>[2x]M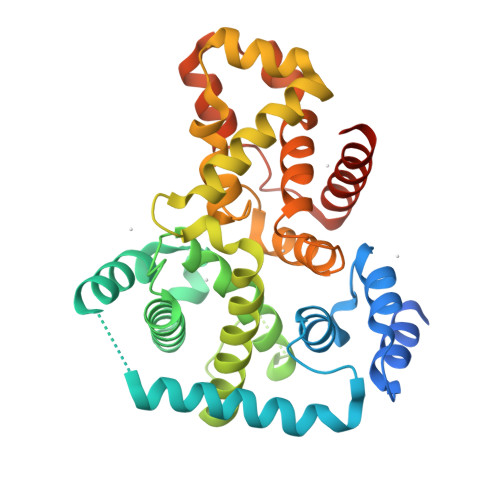HHHHHHSSGRENLYFQGSEREASRLDKFKQLLAGPNTDLEELRRLSWSGIPKPVRPMTWKLLSGYLPANVDRRPATLQRKQKEYFAFIEHYYDSRNDEVHQDTYRQIHIDIPRMSPEALILQPKVTEIFERILFIWAIRHPASGYVQGINDLVTPFFVVFICEYIEAEEVDTVDVSGVPAEVLCNIEADTYWCMSKLLDGIQDNYTFAQPGIQMKVKMLEELVSRIDEQVHRHLDQHEVRYLQFAFRWMNNLLMREVPLRCTIRLWDTYQSEPDGFSHFHLYVCAAFLVRWRKEILEEKDFQELLLFLQNLPTAHWDDEDISLLLAEAYRLKFAFADAPNHYKK>[4x]MSGMEKFKE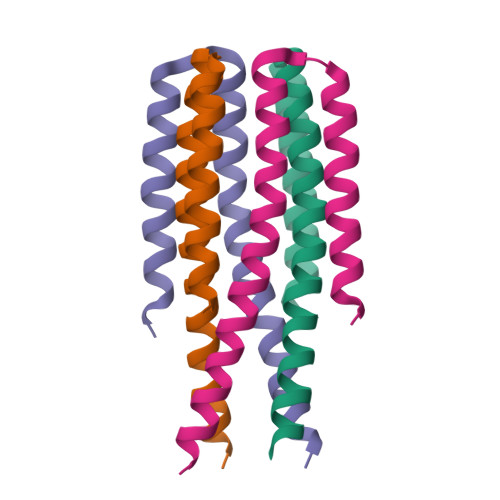QLLEEVKKIVLETMTKVMEHLEKWFVTLAEIIITKSEEKLEELKETMEKSIEELRKEAEGS>[3x]GIEDLIDTAIKNALRVSQPPSTQSTEATSGVNSQEVPALTAVETGASGQAIPSDVVETRHVVNYKTRSESCLESFFGRAACVTILSLTNSSKSGEEKKHFNIWNITYTDTVQLRRKLEFFTYSRFDLEMTFVFTENYPSTASGEVRNQVYQIMYIPPGAPRPSSWDDYTWQSSSNPSIFYMYGNAPPRMSIPYVGIANAYSHFYDGFARVPLEGENTDAGDTFYGLVSINDFGVLAVRAVNRSNPHTIHTSVRVYMKPKHIRCWCPRPPRAVLYRGEGVDMISSAILPLAKVDSITTF;>[3x]SPNVEACGYSDRVRQITLGNSTITTQEAANAIVAYGEWPTYINDSEANPVDAPTEPDVSSNRFYTLESVSWKTTSRGWWWKLPDCLKDMGMFGQNMYYHYLGRSGYTIHVQCNASKFHQGALGVFLIPEFVMACNTESKTSYVSYINANPGERGGEFTNTYNP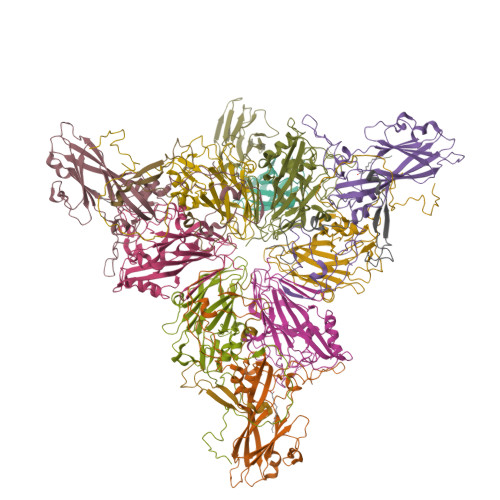SNTDASEGRKFAALDYLLGSGVLAGNAFVYPHQIINLRTNNSATIVVPYVNSLVIDCMAKHNNWGIVILPLAPLAFAATSSPQVPITVTIAPMCTEFNGLRNITVPVHQ;>[3x]GLPTMNTPGSNQFLTSDDFQSPCALPNFDVTPPIHIPGEVKNMMELAEIDTLIPMNAVDGKVNTMEMYQIPLNDNLSKAPIFCLSLSPASDKRLSHTMLGEILNYYTHWTGSIRFTFLFCGSMMATGKLLLSYSPPGAKPPTNRKDAMLGTHIIWDLGLQSSCSMVAPWISNTVYRRCARDDFTEGGFITCFYQTRIVVPASTPTSMFMLGFVSACPDFSVRLLRDTPHISQSKLIGRTQ;>[3x]MGAQVSTQKTGAHENQNVAANGSTINYTTINYYKDSASNSATRQDLSQDPSKFTEPVKDLMLKTAPALN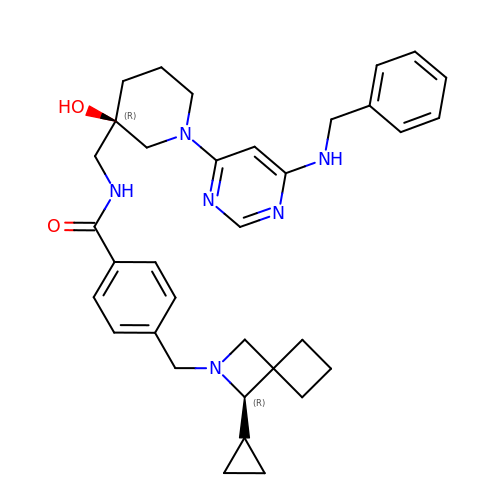4-[[(3R)-3-cyclopropyl-2-azaspiro[3.3]heptan-2-yl]methyl]-N-[[(3R)-3-oxidanyl-1-[6-[(phenylmethyl)amino]pyrimidin-4-yl]piperidin-3-yl]methyl]benzamide | C34 H42 N6 O2 | OWDBESCKAVDZRB-QIKUIUABSA-N> MNTKYNKEFLLYLAGFVDGDGSIIAQIEPNQSYKFKHRLKLTFKVTQKTQRRWFLDKLVDEIGVGYVSDSGSVSNYILSEIKPLHNFLTQL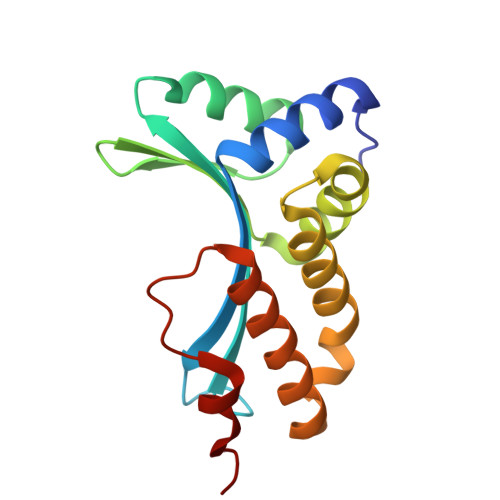QPFLKLKQKQANLVLKIIEQLPSAKESPDKFLEVCTWVDQIAALNDSKTRKTTSETVRAVLD>MMKPEDVIKEQCARAKVVAELWHGFTGGAPKAALENLVVEFNKAQQGRCVRPVPQGGYRDLSTKIKAAFAAGKVPTMAQAFENNIALYLEAKALLPIESLGVKLQGVNLTFLNAVRFGGVVYGVPFNKSIQVLYYNKDLLKKHGVPVPATLEEFVAAAKKLSRAEGGPVYWFQPDASTFAYFFFNLGGSYLKDGKLVLNSKEAVEALTLLQNGVKEGWAKPITSGAINQNLGSGPYAFSVDTSAGYTAYLRAAKFDLGVATLPGRTKGQPGYGLVQGTNLVVFRQASKEEQAVAKDFLEFVLSPRAQA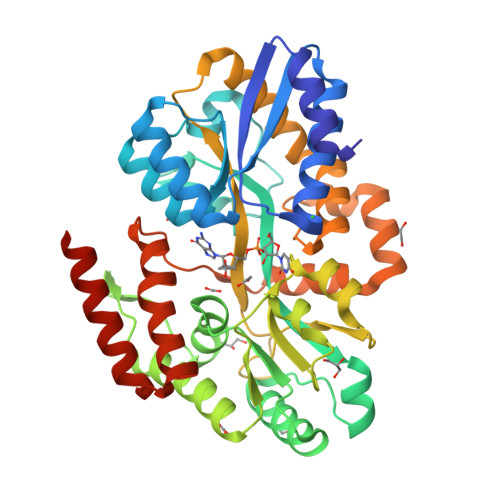VFATATGYVPVTEGALKDPVYQAYAAENPDYATIVRQSRYAKFEPALAEWEQIRFDILGQAIKEAILNKADPKAALDRAQKLAEDLLSSRTRHHHHHH[2x]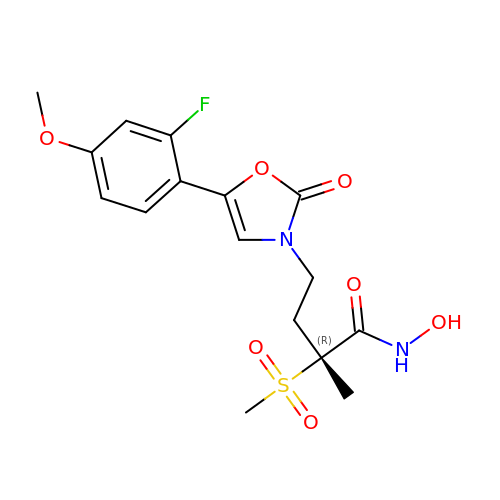(2~{R})-4-[5-(2-fluoranyl-4-methoxy-phenyl)-2-oxidanylidene-1,3-oxazol-3-yl]-2-methyl-2-methylsulfonyl-~{N}-oxidanyl-butanamide | C16 H19 F N2 O7 S | ARJXRYFNKZIMJA-MRXNPFEDSA-N5-fluorocytosine | C4 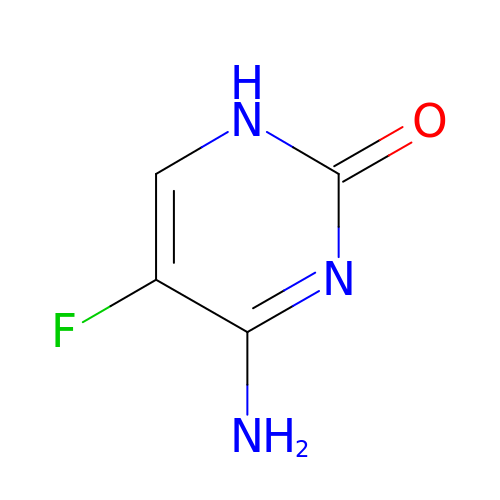H4 F N3 O | XRECTZIEBJDKEO-UHFFFAOYSA-N> MKMKMKLASFGLAAGLAAQVFLPYNALASTEHVTWNQQFQTPQFISGDLLKVNGTSPEELVYQYVEKNENKFKFHENAKDTLQLKEKKNDNLGFTFMRFQQTYKGIPVFGAVVTSHVKDGTLTALSGTLIPNLDTKGSLKSGKKLSEKQARDIAEKDLVANVTKEVPEYEQGKDTEFVVYVNGDEASLAYVVNLNFLTPEPGNWLYIIDAVDGKILNKFNQLDAAKPGDVKSITGTSTVGVGRGVLGDQKNINTTYSTYYYLQDNTRGNGIFTYDAKYRTTLPGSLWADADNQFFASYDAPAVDAHYYAGVTYDYYKNVHNRLSYDGNNAAIRSSVHYSQGYNNAFWNGSQMVYGDGDGQTFIPLSGGIDVVAHELTHAVTDYTAGLIYQNESGAINEAISDIFGTLVEFYANKNPDWEIGEDVYTPGISGDSLRSMSDPAKYGDPDHYSKRYTGTQDNGGVHINSGIINKAAYLISQGGTHYGVSVVGIGRDKLGKIFYRALTQYLTPT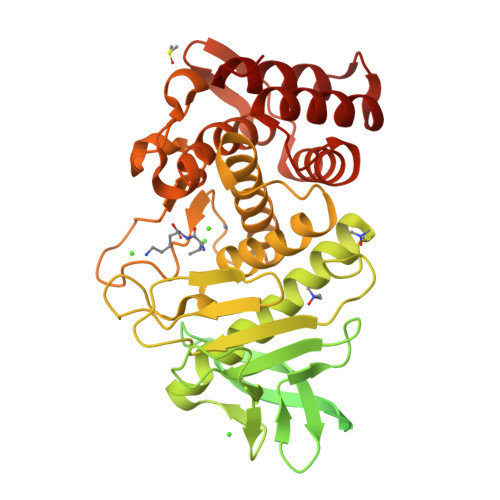SNFSQLRAAAVQSATDLYGSTSQEVASVKQAFDAVGVK> MDYKDDDDKLAAANSSIDLISTSLYKKAGLTMVTGGGAAPPGTVTEPLPSVIVLSAGRKMAAAAAAASGPGCSSAAGAGAAGVSEWLVLRDGCMHCDADGLHSLSYHPALNAILAVTSRGTIKVIDGTSGATLQASALSAKPGGQVKCQYISAVDKVIFVDDYAVGCRKDLNGILLLDTALQTPVSKQDDVVQLELPVTEAQQLLSACLEKVDISSTEGYDLFITQLKDGLKNTSHETAANHKVAKWATVTFHLPHHVLKSIASAIVNELKKINQNVAALPVASSVMDRLSYLLPSARPELGVGPGRSVDRSLMYSEANRRETFTSWPHVGYRWAQPDPMAQAGFYHQPASSGDDRAMCFTCSVCLVCWEPTDEPWSEHERHSPNCPFVKGEHTQNVPLSVTLATSPAQFPCTDGTDRISCFGSGSCPHFLAAATKRGKICIWDVSKLMKVHLKFEINAYDPAIVQQLILSGDPSSGVDSRRPTLAWLEDSSSCSDIPKLEGDSDDLLEDSDSEEHSRSDSVTGHTSQKEAMEVSLDITALSILQQPEKLQWEIVANVLEDTVKDLEELGANPCLTNSKSEKTKEKHQEQHNIPFPCLLAGGLLTYKSPATSPISSNSHRSLDGLSRTQGESISEQGSTDNESCTNSELNSPLVRRTLPVLLLYSIKESDEKAGKIFSQMNNIMSKSLHDDGFTVPQIIEMELDSQEQLLLQDPPVTYIQQFADAAANLTSPDSEKWNSVFPKPGTLVQCLRLPKFAEEENLCIDSITPCADGIHLLVGLRTCPVESLSAINQVEALNNLNKLNSALCNRRKGELESNLAVVNGANISVIQHESPADVQTPLIIQPEQRNVSGGYLVLYKMNYATRIVTLEEEPIKIQHIKDPQDTITSLILLPPDILDNREDDCEEPIEDMQLTSKNGFEREKTSDISTLGHLVITTQGGYVKILDLSNFEILAKVEPPKKEGTEEQDTFVSVIYCSGTDRLCACTKGGELHFLQIGGTCDDIDEADILVDGSLSKGIEPSSEGSKPLSNPSSPGISGVDLLVDQPFTLEILTSLVELTRFETLTPRFSATVPPCWVEVQQEQQQRRHPQHLHQQHHGDAAQHTRTWKLQTDSNSWDEHVFELVLPKACMVGHVDFKFVLNSNITNIPQIQVTLLKNKAPGLGKVNALNIEVEQNGKPSLVDLNEEMQHMDVEESQCLRLCPFLEDHKEDILCGPVWLASGLDLSGHAGMLTLTSPKLVKGMAGGKYRSFLIHVKAVNERGTEEICNGGMRPVVRLPSLKHQSNKGYSLASLLAKVAAGKEKSSNVKNENTSGTRKSENLRGCDLLQEVSVTIRRFKKTSISKERVQRCAMLQFSEFHEKLVNTLCRKTDDGQITEHAQSLVLDTLCWLAGVHSNGPGSSKEGNENLLSKTRKFLSDIVRVCFFEAGRSIAHKCARFLALCISNGKCDPCQPAFGPVLLKALLDNMSFLPAATTGGSVYWYFVLLNYVKDEDLAGCSTACASLLTAVSRQLQDRLTPMEALLQTRYGLYSSPFDPVLFDLEMSGSSCKNVYNSSIGVQSDEIDLSDVLSGNGKVSSCTAAEGSFTSLTGLLEVEPLHFTCVSTSDGTRIERDDAMSSFGVTPAVGGLSSGTVGEASTALSSAAQVALQSLSHAMASAEQQLQVLQEKQQQLLKLQQQKAKLEAKLHQTTAAAAAAASAVGPVHNSVPSNPVAAPGFFIHPSDVIPPTPKTTPLFMTPPLTPPNEAVSVVINAELAQLFPGSVIDPPAVNLAAHNKNSNKSRMNPLGSGLALAISHASHFLQPPPHQSIIIERMHSGARRFVTLDFGRPILLTDVLIPTCGDLASLSIDIWTLGEEVDGRRLVVATDISTHSLILHDLIPPPVCRFMKITVIGRYGSTNARAKIPLGFYYGHTYILPWESELKLMHDPLKGEGESANQPEIDQHLAMMVALQEDIQCRYNLACHRLETLLQSIDLPPLNSANNAQYFLRKPDKAVEEDSRVFSAYQDCIQLQLQLNLAHNAVQRLKVALGASRKMLSETSNPEDLIQTSSTEQLRTIIRYLLDTLLSLLHASNGHSVPAVLQSTFHAQACEELFKHLCISGTPKIRLHTGLLLVQLCGGERWWGQFLSNVLQELYNSEQLLIFPQDRVFMLLSCIGQRSLSNSGVLESLLNLLDNLLSPLQPQLPMHRRTEGVLDIPMISWVVMLVSRLLDYVATVEDEAAAAKKPLNGNQWSFINNNLHTQSLNRSSKGSSSLDRLYSRKIRKQLVHHKQQLNLLKAKQKALVEQMEKEKIQSNKGSSYKLLVEQAKLKQATSKHFKDLIRLRRTAEWSRSNLDTEVTTAKESPEIEPLPFTLAHERCISVVQKLVLFLLSMDFTCHADLLLFVCKVLARIANATRPTIHLCEIVNEPQLERLLLLLVGTDFNRGDISWGGAWAQYSLTCMLQDILAGELLAPVAAEAMEEGTVGDDVGATAGDSDDSLQQSSVQLLETIDEPLTHDITGAPPLSSLEKDKEIDLELLQDLMEVDIDPLDIDLEKDPLAAKVFKPISSTWYDYWGADYGTYNYNPYIGGLGIPVAKPPANTEKNGSQTVSVSVSQALDARLEVGLEQQAELMLKMMSTLEADSILQALTNTSPTLSQSPTGTDDSLLGGLQAANQTSQLIIQLSSVPMLNVCFNKLFSMLQVHHVQLESLLQLWLTLSLNSSSTGNKENGADIFLYNANRIPVISLNQASITSFLTVLAWYPNTLLRTWCLVLHSLTLMTNMQLNSGSSSAIGTQESTAHLLVSDPNLIHVLVKFLSGTSPHGTNQHSPQVGPTATQAMQEFLTRLQVHLSSTCPQIFSEFLLKLIHILSTERGAFQTGQGPLDAQVKLLEFTLEQNFEVVSVSTISAVIESVTFLVHHYITCSDKVMSRSGSDSSVGARACFGGLFANLIRPGDAKAVCGEMTRDQLMFDLLKLVNILVQLPLSGNREYSARVSVTTNTTDSVSDEEKVSGGKDGNGSSTSVQGSPAYVADLVLANQQIMSQILSALGLCNSSAMAMIIGASGLHLTKHENFHGGLDAISVGDGLFTILTTLSKKASTVHMMLQPILTYMACGYMGRQGSLATCQLSEPLLWFILRVLDTSDALKAFHDMGGVQLICNNMVTSTRAIVNTARSMVSTIMKFLDSGPNKAVDSTLKTRILASEPDNAEGIHNFAPLGTITSSSPTAQPAEVLLQATPPHRRARSAAWSYIFLPEEAWCDLTIHLPAAVLLKEIHIQPHLASLATCPSSVSVEVSADGVNMLPLSTPVVTSGLTYIKIQLVKAEVASAVCLRLHRPRDASTLGLSQIKLLGLTAFGTTSSATVNNPFLPSEDQVSKTSIGWLRLLHHCLTHISDLEGMMASAAAPTANLLQTCAALLMSPYCGMHSPNIEVVLVKIGLQSTRIGLKLIDILLRNCAASGSDPTDLNSPLLFGRLNGLSSDSTIDILYQLGTTQDPGTKDRIQALLKWVSDSARVAAMKRSGRMNYMCPNSSTVEYGLLMPSPSHLHCVAAILWHSYELLVEYDLPALLDQELFELLFNWSMSLPCNMVLKKAVDSLLCSMCHVHPNYFSLLMGWMGITPPPVQCHHRLSMTDDSKKQDLSSSLTDDSKNAQAPLALTESHLATLASSSQSPEAIKQLLDSGLPSLLVRSLASFCFSHISSSESIAQSIDISQDKLRRHHVPQQCNKMPITADLVAPILRFLTEVGNSHIMKDWLGGSEVNPLWTALLFLLCHSGSTSGSHNLGAQQTSARSASLSSAATTGLTTQQRTAIENATVAFFLQCISCHPNNQKLMAQVLCELFQTSPQRGNLPTSGNISGFIRRLFLQLMLEDEKVTMFLQSPCPLYKGRINATSHVIQHPMYGAGHKFRTLHLPVSTTLSDVLDRVSDTPSITAKLISEQKDDKEKKNHEEKEKVKAENGFQDNYSVVVASGLKSQSKRAVSATPPRPPSRRGRTIPDKIGSTSGAEAANKIITVPVFHLFHKLLAGQPLPAEMTLAQLLTLLYDRKLPQGYRSIDLTVKLGSRVITDPSLSKTDSYKRLHPEKDHGDLLASCPEDEALTPGDECMDGILDESLLETCPIQSPLQVFAGMGGLALIAERLPMLYPEVIQQVSAPVVTSTTQEKPKDSDQFEWVTIEQSGELVYEAPETVAAEPPPIKSAVQTMSPIPAHSLAAFGLFLRLPGYAEVLLKERKHAQCLLRLVLGVTDDGEGSHILQSPSANVLPTLPFHVLRSLFSTTPLTTDDGVLLRRMALEIGALHLILVCLSALSHHSPRVPNSSVNQTEPQVSSSHNPTSTEEQQLYWAKGTGFGTGSTASGWDVEQALTKQRLEEEHVTCLLQVLASYINPVSSAVNGEAQSSHETRGQNSNALPSVLLELLSQSCLI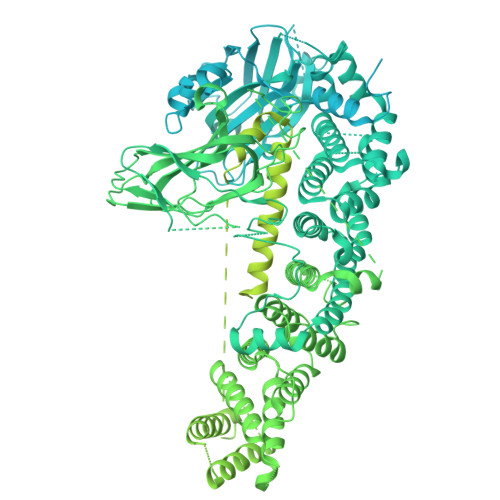PAMSSYLRNDSVLDMARHVPLYRALLELLRAIASCAAMVPLLLPLSTENGEEEEEQSECQTSVGTLLAKMKTCVDTYTNRLRSKRENVKTGVKPDASDQEPEGLTLLVPDIQKTAEIVYAATTSLRQANQEKKLGEYSKKAAMKPKPLSVLKSLEEKYVAVMKKLQFDTFEMVSEDEDGKLGFKVNYHYMSQVKNANDANSAARARRLAQEAVTLSTSLPLSSSSSVFVRCDEERLDIMKVLITGPADTPYANGCFEFDVYFPQDYPSSPPLVNLETTGGHSVRFNPNLYNDGKVCLSILNTWHGRPEEKWNPQTSSFLQVLVSVQSLILVAEPYFNEPGYERSRGTPSGTQSSREYDGNIRQATVKWAMLEQIRNPSPCFKEVIHKHFYLKRVEIMAQCEEWIADIQQYSSDKRVGRTMSHHAAALKRHTAQLREELLKLPCPEGLDPDTDDAPEVCRATTGAEETLMHDQVKPSSSKELPSDFQL12-AMINO-DODECANOIC ACID | C12 H25 N O2 | 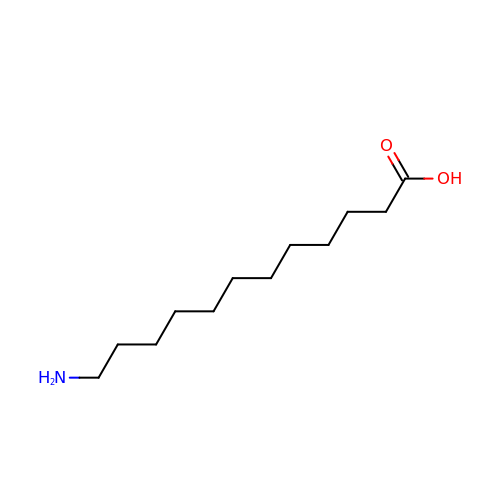PBLZLIFKVPJDCO-UHFFFAOYSA-N> MLLPLLLLLPMCWAVEVKRPRGVSLTNHHFYDESKPFTCLDGSATIPFDQVNDDYCDCKDGSDEPGTAACPNGSFHCTNTGYKPLYIPSNRVNDGVCDCCDGTDEYNSGVICENTCKEKGRKERESLQQMAEVTREGFRLKKILIEDWKKAREEKQKKLIELQAGKKSLEDQVEMLRTVKEEAEKPEREAKEQHQKLWEEQLAAAKAQQEQELAADAFKELDDDMDGTVSVTELQTHPELDTDGDGALSEAEAQALLSGDTQ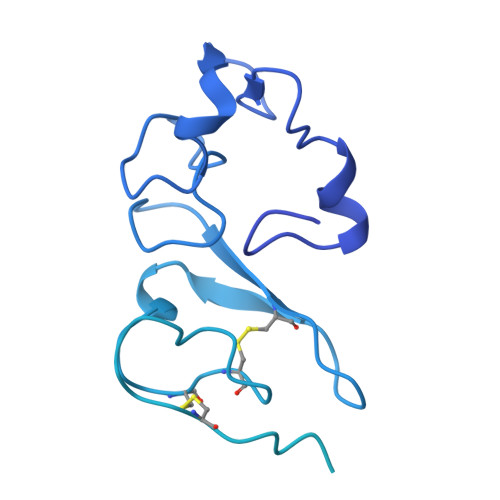TDATSFYDRVWAAIRDKYRSEALPTDLPAPSAPDLTEPKEEQPPVPSSPTEEEEEEEEEEEEEAEEEEEEEDSEEAPPPLSPPQPASPAEEDKMPPYDEQTQAFIDAAQEARNKFEEAERSLKDMEESIRNLEQEISFDFGPNGEFAYLYSQCYELTTNEYVYRLCPFKLVSQKPKLGGSPTSLGTWGSWIGPDHDKFSAMKYEQGTGCWQGPNRSTTVRLLCGKETMVTSTTEPSRCEYLMELMTPAACPEPPPEAPTEDDHDEL> MSSGKKPVKV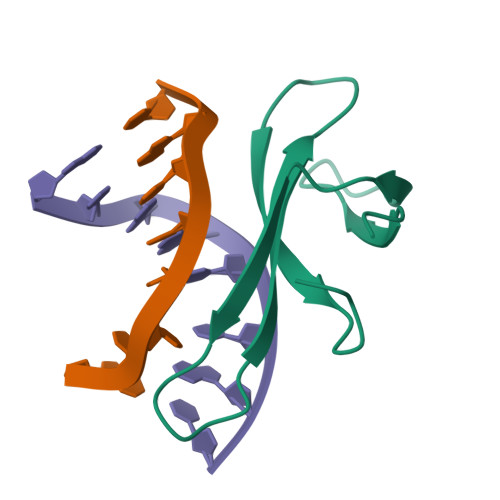KTPAGKEAELVPEKVWALAPKGRKGVKIGLFKDPETGKYFRHKLPDDYPI>[6x]MDTLLILGDSLSAGYRMSASAAWPALLNDKWQSKTSVVNASISGDTSQQGLARLPALLKQH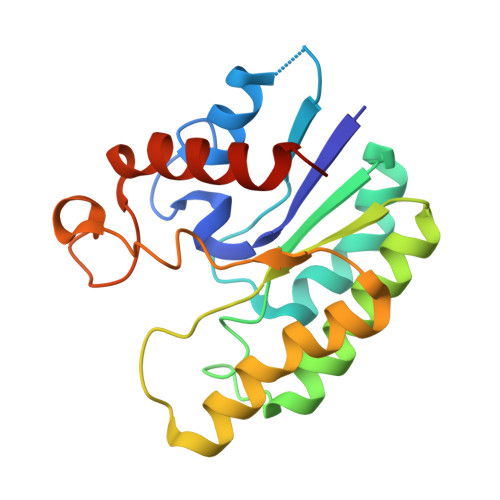QPRWVLVELGGNDGLRGFQPQQTEQTLRQILQDVKAANAEPLLMQIRLPANYGRRYNEAFSAIYPKLAKEFDVPLLPFFLDEVGLKPQWMQDDGIHPNRDAQPFIADWMAKQLQPLVNHDS> TYMNNTEAICDAKGFAPFSKDNGIRIGSRGHIFVIREPFV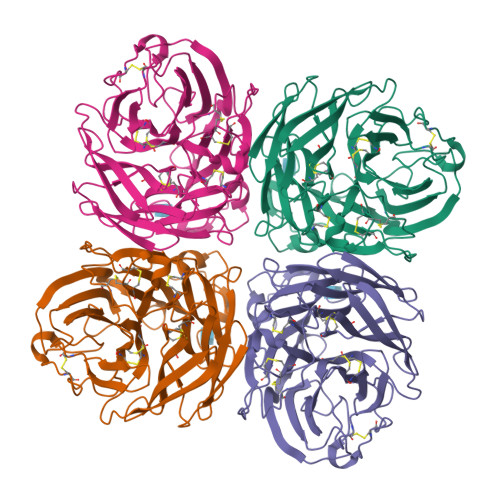SCSPIECRTFFLTQGSLLNDKHSNGTVKDRSPFRTLMSVEVGQSPNVYQARFEAVAWSATACHDGKKWMTVGVTGPDSKAVAVIHYGGVPTDVVNSWAGDILRTQESSCTCIQGDCYWVMTDGPANRQAQYRIYKANQGRIIGQTDISFNGGHIEECSCYPNDGKVECVCRDGWTGTNRPVLVISPDLSYRVGYLCAGIPSDTPRGEDTQFTGSCTSPMGNQGYGVKGFGFRQGTDVWMGRTISRTSRSGFEILRIKNGWTQTSKEQIRKQVVVDNLNWSGYSGSFTLPVELSGKDCLVPCFWVEMIRGKPEEKTIWTSSSSIVMCGVDYEVADWSWHDGAILPFDIDKM>GPKYTMFHYLRAQEFEHGKSRIALTNSVNEALLNPSRVYTFFSSDYVKKVNKATEAAMFLGWVEQLVYDFTDETSEVSTTDKIADITIIIPYIGPALNIGNMLYKDDFVGALIFSGAVILLEFIPEIAIPVLGTFALVSYIANKVLTVQTIDNALSKRNEKWDEVYKYIVTNWLAKVNTQIDLIRKKMKEALENQAEATKAIINYQYNQYTEEEKNNINFNIDDLSSKLNESINKAMININKFLNQCSVSYLMNSMIPYGVKRLEDFDASLKDALLKYIYDNRGTLIGQVDRLKDKVNNTLSTDIPFQLSKYVDNQRLLSTFTEYIK[2x]

Botulinum neurotoxins (BoNTs), the most poisonous biological toxins for mammals, are speculated to exploit a similar mechanism to block neurotransmitter release at neuromuscular junctions that results in fatal botulism. A BoNT molecule consists of a light chain (LC) and a heavy chain (HC) that are linked by a disulfide bridge. LC is a zinc-dependent endopeptidase that is delivered into the cytosol where it degrades SNARE proteins to inhibit synaptic vesicle exocytosis. Membrane translocation of LC is mediated by HC, which can be subdivided into a translocation domain (HN) and a receptor-binding domain (HC).

To better understand how acidic pH triggers membrane insertion of tHNA, we crystallized tHNA at pH 5.1 and determined the structure at 2.7 Å resolution. Two molecules of tHNA form a homodimer in the asymmetric unit. However, we observed a major conformational change in a central helical bundle (residues E620–F667) of HN. At acidic pH, the αA protrudes outward to form the center of the β2/β3 hairpin. This leaves the hydrophobic groove exposed to solvent, thus helices αB and αC transform into the β4/β5 hairpin to partly shield the solvent-exposed surface. The low pH conformation is facilitated by several non-polar residues (V653, F658, and F667). These residues are solvent-exposed at neutral pH, but flip inward at acidic pH. Notably, the highly conserved Y636 that is important for stabilizing the local structure at neutral pH flips out to be solvent exposed at acidic pH. Specifically, the tHNA homodimer forms a two-side flattened β-barrel that is stabilized by swapping the β2/β3 hairpin between the two protomers, which forms an antiparallel β sheet with β1, β4, and β5. As a result, most of the exposed hydrophobic side-chains of the β-hairpins are buried within the tHNA homodimer in the crystal structure.>[4x]MQRGSAYFLRGRARQNLKVLLLYCAFLLVMLLAYASIFRYLMWHLEGRAYSFMAGIYWTITVMTTLGFGDITFESDAGYLFASIVTVSGVIFLDIILPFGFVSMFLAPWIERRLRYHPTIELPDDTRGHILIFGIDPITRTLIRKLESRNHLFVVVTDNYDQALHLEEQEGFKVVYGSPTDAHVLAGLRVAAARSIIANLSDPDNANLCLTVRSLCQTPIIAVVKEPVHGELLRLAGANQVVPLTRILGRYLGIRATTCGALAHILDSFGNLQIAELPVHGTPFAGKTIGESGIRQRTGLSIIGVWERGSLTTPQRETVLTEQSLLVLAGTKSQLAALEYLIGEAPEDELIFIIGHGRIGCAAAAFLDRKPVPFILIDRQESPVCNDHVVVYGDATVGQTLRQAGIDRASGIIVTTNDDSTNIFLTLACRHLHSHIRIVARANGEENVDQLYAAGADFVVSNASVGANILGNLLEHKESAFLSEGMAVFRRPLPPAMAGKTIAETRLRPLTGCSIVAIEAPDRADILISPPPETILAEGARLILIGTSEQEKTFDQTIAARLVPR

Each GsuK subunit contains two tandem RCK domains, reminiscent of Slo K+ channels. We demonstrate that GsuK is a nucleotide-activated and Ca2+-deactivated K+ channel and reveal the structural mechanism of multi-ligand gating of this double-RCK K+ channel and a distinct pore opening mechanics. Ca2+ stabilizes the closed gating ring by binding at the inter-subunit assembly interfaces and deactivates the GsuK channel. While both NAD+ and ADP anchor their adenine rings at the same site on RCK2 by using the conserved nucleotide binding motif, they utilize different functional groups and activate the channel at different sites.

Giant liposome patching was employed to assay the functional properties of both wild-type GsuK and L97D pore mutant, a mutation that enhances the channel conductance and open probability, and also yields better diffracting crystals (‘Materials and methods’). Two full-length channel structures, wild-type channel and L97D mutant, were determined at 3.7 Å and 2.6 Å, respectively. Both channels share a similar overall structure and, therefore, the higher resolution L97D mutant is used here for the description of the overall full-length channel structure. The L97D mutant channel crystals are of the space group C2 with unit cell dimensions of a = 232.9 Å, b = 111.7 Å, c = 164.1 Å and β = 134.5°, and contain four channel subunits in an asymmetric unit. These subunits do not belong to the same channel tetramer and, instead, are divided into two half channels, which participate in the formation of two channel tetramers with their crystallographic twofold related partners. The gating ring of the full-length channel tetramer adopts a similar structure to the isolated gating ring, indicating a closed conformation. In the L97D mutant, a noticeable helix bend occurs at Gly92 (hinge 1), whereas a sharp turn occurs between TM2B and 2C (hinge 2) in the wild-type channel inner helix. The L97D mutant appears to promote inner helix bending at the glycine gating hinge (Gly92) and the direction of the helix bend is parallel with the orientation of the linker between the pore and the gating ring. Its gating ring, however, is still in the Ca2+-bound, closed conformation, which locks the intracellular gate closed at the end of the inner helix and prevents the concurrent movement of the TM2C with TM2B. Consequently, the sharp turn between TM2B and 2C in the wild-type channel inner helix becomes straightened in the L97D mutant. These structural differences, along with the electrophysiological observation that the L97D mutant favors pore opening and has lower sensitivity to Ca2+ deactivation, suggest that the L97D structure is in an intermediate state in which the pore inner helices are undergoing conformational changes towards opening but the channel's intracellular gate remains shut, deactivated by Ca2+.> IPCGESCVWGPCISSAIGCSCKSKVCY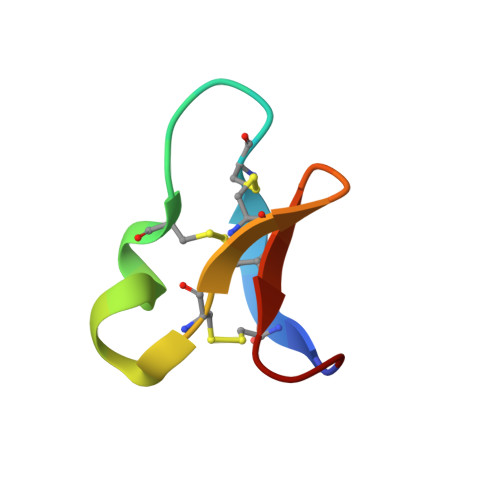RNG>MSNKLRLCQVASVKDGEPVAVYQEKMPALAVYNVDGEVFVTDNLCTHGNAMLTDGYQDGTIIECPFHGGSFDIATGAAKAFPCQIPIKTYPVTIEDGWVCIDQPKESA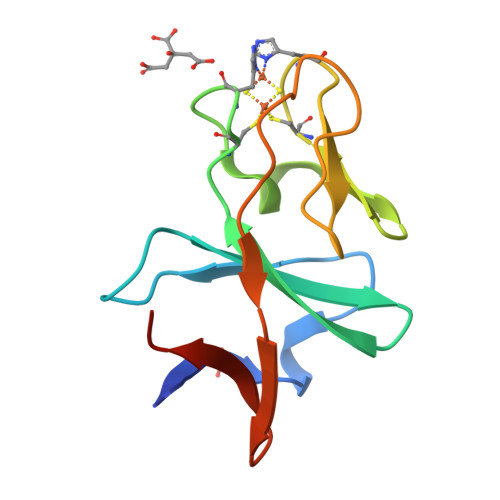[2x]> MFQQLSARLQEAIGRLRGRGRITEEDLKATLREIRRALMDADVNLEVARDFVERVREEALGKQVLESLTPAEVILATVYEALKEALGGEARLPVLKDRNLWFLVGLQGSGKTTTAAKLALYYKGKGRRPLLVAADTQRPAAREQLRLLGEKVGVPVLEVMDGESPESIRRRVEEKARLEARDLILVDTAGRLQIDEPLMGELARLKEVLGPDEVLLVLDAMTGQEALSVARAFDEKVGVTGLVLTKLDGDARGGAALSARHVTGK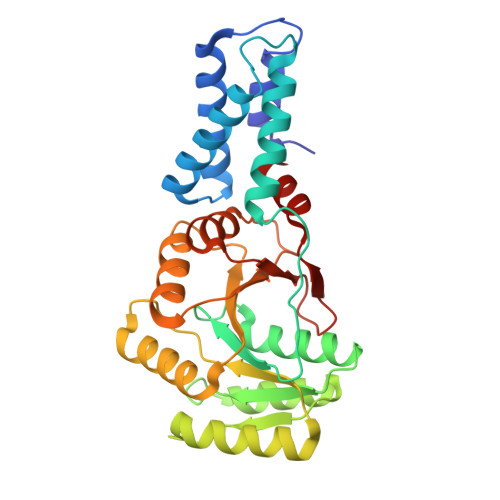PIYFAGVSEKPEGLEPFYPERLAGRILGM>[2x]LVPRGSHMAKKVRFYRNGDRYFKGIV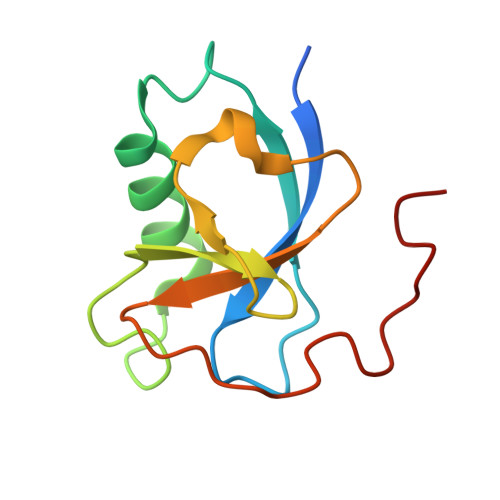YAVSSDRFRSFDALLADLTRSLSDNINLPQGVRYIYTIDGSRKIGSMDELEEGESYVCSSDNFFDDVEYTKNVNPNWSVN>TYSTLTMDRLESLIKEHSIIDDNYIKTLLVIKNLMLKDNLDTLAMVRGLNVKIRKAFKATYGYNYNYIKLTEYLSIIF[3x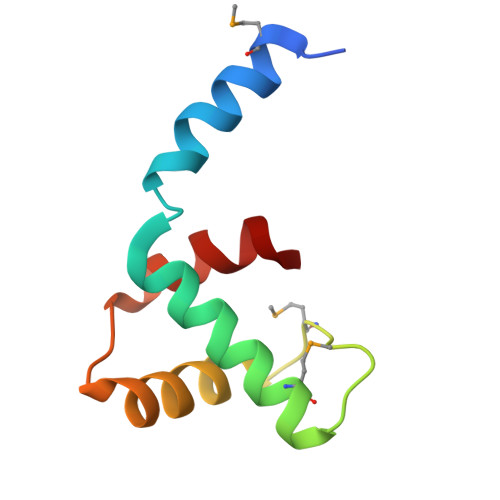]>EEFMARAISAIAELAKKAIEAIYRLADNHTTDTFMAKAIEAIAELAKEAIKAIADLAKNHTTEEFMARAISAIAELARKAIDAIYRLARNHTTDTFMAKAIEAIAELAKEAIKAIADLAKNHTTEDFMDEAISAIAELARKAIEAILRLASNLTSETYMRKAQEAIEKIARTAEEAIRDLARNLEDQERRERAKSARDEIKRFAEDARKKIEVLALLKRSREYLKKVALIQLVIAFVFLILLILLSWRSEELIRELEEKGAASEAELARMKQQHMTAYLQAALTAWEIISKSVIALLLLQQNQL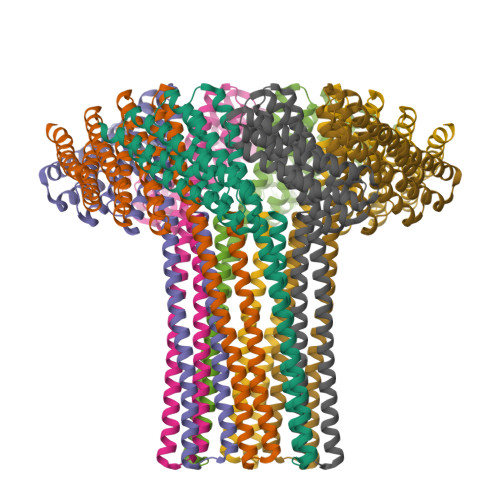NLELRH[8x]>MDVNNSKPNDYGTLVKIEQKLFNNANTLKTTTPIKHVVIIFQENNSFDRYFGMYPNAKNPEGEPKFVAKENTPNVNGLTKQLLENNPNTKNPYRLDRNFQPCSQNHEYHQEISSFNGGLMNKFVEHGGHDNDTYKQNCDGQVMGYYDGNTVTALWNYAQNFALNDNTFGTTFGPSTPGALNLVAGANGPAMSPSGNLENIENNYIIDDPNPYYDDCSYGTSKSGDTNTAVAKITDGYNIGHYLTQKGITWGWFQGGFKPTSYSGKTAICDAMSTNKFGVKSRDYIPHHEPFNYWKETSNPHHLAPSDDKYIGSNDQANHQYDISEFWKALDQNNMPAVSYLKAPGYQDGHGGYSNPLDEQEWLVNTINRIQQSKDWDSTAIIIIYDDSDGDYDHVYSPKSQFSDIKGRQGYGPRLPMLVISPYAKANYVDHSLLNQASVLKFIEYNWGIGSVSKYSNDKYSNNILNMFDFN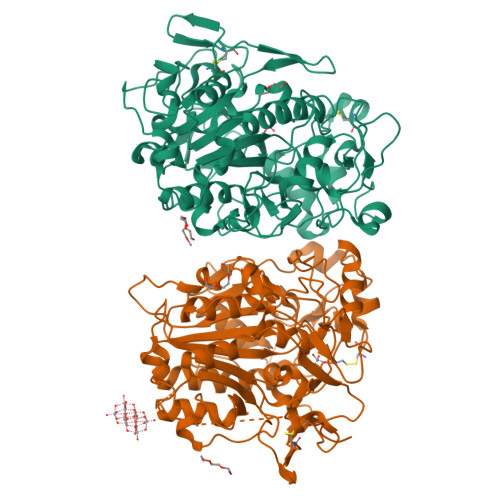KEQKTLKLILDPKTGLVMDKLNHHHHH[2x]> MKGKLTGKDKLIVDEFEELGEQESDIDEFDLLEGDEKLPGDSELDKTTSIYPPETSWEVNKGMNSSRLHKLYSLFFDKSSAFYLGDDVSVLEDKPLTGAYGFQSKKNDQQIFLFRPDSDYVAGYHVDAKSDAGWVNDKLDRRLSEISEFCSKATQPATFILPFVEMPTDITKGVQHQVLLTISYDPKSKQLTPTVYDSIGRDTYSESLSSYFKGKYRTTCDEILTQSIEKAIKSTDFTLGKFTRAAYNHQNRLTEGNSGSYTFRTIKEVISSSAQGTEVKIPGSGYITSNSYLTSQHVQDIESCIKYRNLGVVDIESALTEGKTLPVQLS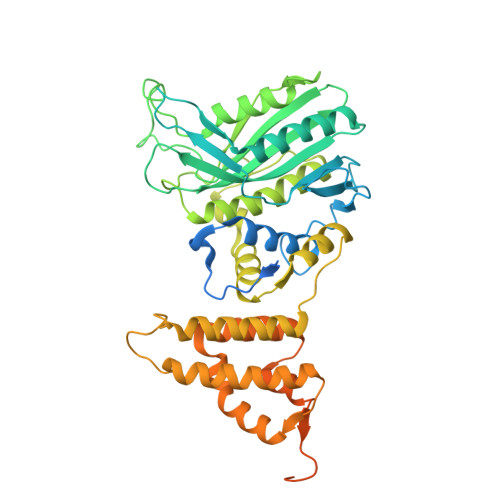EFIVALEDYGKLRSQQSEKSMLNFIGYSKTAKLTAVELLIGILNDIKGKNEISESQYDKLVKEVDCLMDSSLGKLVQFHLKNLGAESLQKLVLPCVKFDDTIDDFVTIEKDELFDVPDITGEELASKKGIEQGALDKEALLKQKQIKTDLLDLREEDKTGLKKPLHGGIKVK> TKPYSSPPTNLRSLRDRLTQVAERQGVVFGRLQRHVAMIVVAQFAATLTDDTGAPLLLVKGGSSLELRRGIPDSRTSKDFDTVARRDIELIHEQLADAGETGWEGFTAIFTAPEEIDVPGMPVKPRRFTAKLSYRGRAFATVPIEVSSVEAGNADQFDTLTSDALGLVGVPAAVAVPCMTIPWQIAQKLHAVTAVLEEPKVNDRAHDLVDLQLLEGLLLDADLMPTRSACIAIFEARAQHPWPPRVATLPHWPLIYAGALEGLDHLELARTVDAAAQAVQRFVARIDRATKR

The Mycobacterium tuberculosis NTase toxin family, MenT, modifies tRNAs to block translation. MenT toxin activity can be stringently regulated by diverse MenA antitoxins. MenT and AbiEii toxins share four highly conserved NTase motifs scattered throughout their structures, proposed to facilitate co-ordination of metals (motifs I and II), base stacking, and transfer of nucleotides to tRNA isoacceptors (motif III), and to contribute to catalysis (motif IV). Our study reveals a conserved mechanism for the control of tuberculosis toxins, and demonstrates how active site auto-phosphorylation can regulate the activity of widespread NTases.

Recent characterization of the MenAT1 and MenAT3 TA systems found that MenA1 binds asymmetrically to two MenT1 toxin protomers to form a stable heterotrimeric complex in vitro, whereas MenA3 appears to function as a kinase, phosphorylating MenT3 at the highly conserved catalytic S786,21. We first sought to establish whether phosphorylation of MenT3 S78 results in steric occlusion of the conserved NTase cavity, as had been observed for MenT1 and MenT1-p. Structural alignment of respective protein backbones returned an RMSD of 0.144 Å (268 atoms), and there was some small movement of the S78 loop, leading to occlusion of the active site by the phosphoserine (SEP), albeit to a lesser extent than we observed for MenT1-p. Using the solved crystal structure of MenT3 as a starting model, we performed MD simulations of ATP and Mg2+ binding in the absence and presence of MenA3 to establish whether a conformational change to the S78-bearing loop ensued. In the absence of antitoxin, R76 and K79 stabilize the γ-phosphate of ATP, which lies 10.0 Å from the sidechain of S78. This arrangement closely resembles the protein-ligand interactions observed for the MenT1-ATP pose. H207 and K189 interact with the β-phosphate, whilst R205 directly interacts with the α-phosphate, and the only non-phosphate interaction is formed between the ribose 2′ OH and R238. When docked to the Alphafold-predicted MenA3:MenT3 heterodimer used to run the simulations (pTM score 0.84), the looped region of MenA3 connecting α5-β4, spanning residues H98-I108, forces MenT3 S78 into an inwards-facing conformation akin to binding of MenA1 to MenT1. As a result, the overall distance between S78 and the terminal phosphate of ATP is reduced to 3.1 Å. We therefore conclude that regulation of MenT1 and MenT3 NTases occurs by antitoxin-induced toxin auto-phosphorylation.> MSGQFTGTGTGGDVFKVDLNEQFDRADMVWIGTASVLVWIMIPGVGLLYSGISRKKHALSLMWAALMAACVAAFQWFWWGYSLVFAHNGSVFLGTLQNFCLKDVLGAPSIVKTVPDILFCLYQGMFAAVTAILMAGAGCERARLGPMMVFLFIWLTVVYCPIAYWTWGGNGWLVSLGALDFAGGGPVHENSGFAALAYSLWLGKRHDPVAKGKVPKYKPHSVSSIVMGTIFLWFGWYGFNGGSTGNSSMRSWYACVNTNLAAATGGLTWMLVDWFRTGGKWSTVGLCMGAIAGLVGITPAAGYVPVYTSVIFGIVPAIICNFAVDLKDLLQIDDGMDVWALHGVGGFVGNFMTGLFAADYVAMIDGTEIDGGWMNHHWKQLGYQLAGSCAVAAWSFTVTSIILLAMDRIPFLRIRLHEDEEMLGTDLAQIGEYAYYADDD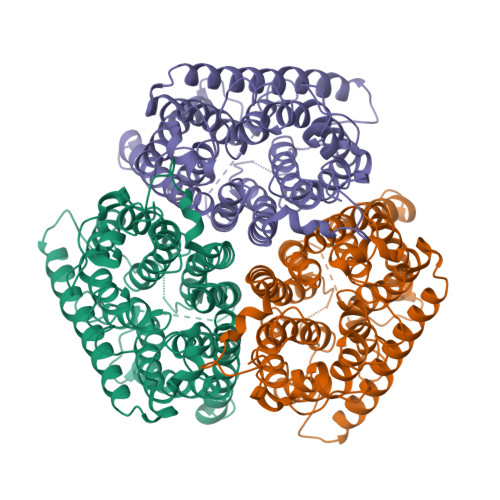PEHHHHHH> MSINTAHTQDGLGVVLFYGERLLVTYDGCKLTLSGSGQQPNGKYSGTAYLTSHRVIFLSKDRSAALNSLSMPFVFMARVAIKAPTFGPNHIEGFVSSEAGQWSGEMPFKLVFNHGGAIEFGKSLLELGTRASKLQNSYKTPAAPPLCEIYACPPPAYTPFV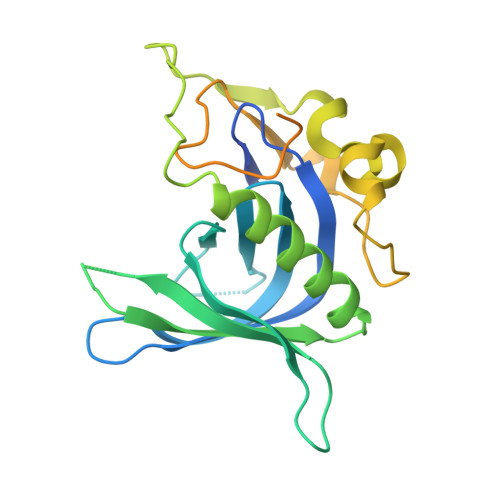NDPYYNSFMQPHPSFSPPPADYLYQTNSPPPYPGAVPPPYTANPGPPPPYTAAAASSMPPYPTGGPPPVNTAYYYPSDPNTFYAPPYSQASAPPMEPEDKKNL> MRKYLEEKYNKFSLRKLTVGVCSMTIGSFFLVSTVQPEDYVVKAADNAIVHYKYVGEDNLTDKEKELIKKEVPSVVSSKEETYYLVFKPTKTTQLNKLPNTGLNYGVGSMLLGGMLGLVVVVVAKGKNKSRKILSILLVTSLGATTLELPARAMEDLQLSVYNMDYNLKVGDKLPEISSIPGYSFVGFIKNEAETKKENEEVKEQITSQQHNKKQPELKENTDENVIENKQENKTTLKISDKKEDKKVIENINKKDEKKVQGVNTVNPQDEVLAGKLTKPELLYSDKIIETPLKYNQIIESNDQLPEGTTRIKQQGKEGKKTEVIRMFTVEGKEVSRELISTKTEEPVSEIIEKGTKKAVSNVITKGQKLVKPAVEVKPEYTGVQAGAIVEPVKAEVPKEYTGVQAGAIVEPAKVETPKEYTGVQAGAIVEPAKAEVSKEYTGVQAGTIVEPAKAEVPKEYTGVQAGAIVEPEKVEPQYGGVTSGALVKPEKIEAPKEYTGVQAGAVVEPAKAEAPKEYRGVQAGAIVEPEKIESPKEYTGVQAGAVVEPAKAEVPKEYRGVQAGAIVEPEKIESPKEYTGEQSGAIVEPEKVETTKEYTGIQAGALVEPEKVEAPKEYTGVQAGAIVEPEKVEPPKEYTGVQAGAIVEPEKVEAPKEYTGKIEPLKTENPKPTVENNNTAEINNVPKNASALLRMNFVKGNQVLSGTGSATFIAPNVLLTVAHNFINNSADNSTGEFIGDKSKNTYEWQTPDGQKGSFTSEDIHFYNKKDYPKGFIYDLAVITLPQSTRRQHANLVENYSKVNVNDKLNVYGYPRGEYAHLKDTTVEIEQKYANNTYGVQYQGGKAGMSGGGIFNSKGEVIGLHQNGAENRSGGLILSPTQLDWIRSIIKGKEITPNYDALERHKDEKKDDIKEEKQVDKKLELRNISNVELYTLENNKYRHVSSLSSVPTNPEAYFMKVKSENFKDVMLPVKSIESARKDNQDVYKIVGQANDLIQHENNITLENYTYYLPKTVNSENGVYTSFKNLVDAMNINPYGTFRLGATMDAREVELSDGQESYINKEFSGKLIGENKGKYYAIYNLKKPLFKALSHATIQDLSIKEANVSSKEDAATIAKEAKNDTTIANVHSSGVIAGERSIGGLISQVTDSTISNSSFTGRITNTYDTTATYQIGGLVGKLSGVGALIEKSISSIDMATNANTGDQVVGGVAGVVDKKATIRNSYVEGNLNNVKPFGKVGGVVGNLWDRETSEVSNSGNLTNVLSDVNVTNGNAIAGYDFNGIKATNTYSNKNNKVVKVVQVDDEVLSKDSEEQRGTVLENNIVLEKKIELVPKKNTKIEDFNFSSRYETDYKNLKDADVSRLRVYKNIEKLLPFYNRETIVKYGNLVDANNTLYTKDLVSVVPMKDKEVISDINKNKTSINKLLLHYSDNTSQTLDIKYLQDFSKVAEYEIANTKLIYTPNTLLHSYNNIVKAVLNDLKSVQYDSDAVRKVLDISSNIKLTELYLDEQFTKTKANIEDSLSKLLSADAVIAENSNSIIDNYVIEKIKNNKEALLLGLTYLERWYNFKYDNTSAKDLVLYHLDFFGKSNSSALDNVIELGKSGFNNLLAKNNVITYNVLLSKNYGTEGLFKALEGYRKVFLPNVSNNDWFKTQSKAYIVEEKSTIPEVSSKQSKQGTEHSIGVYDRLTSPSWKYQSMVLPLLTLPEEKMIFMIANISTIGFGAYDRYRSSEYPKGDKLNRFVEENAQAAAKRFRDHYDYWYKILDKENKEKLFRSVLVYDAFRFGNDTNKETQEANFETNNPVIKNFFGPAGNNVVHNKHGAYATGDAFYYMAYRMLDKSGAVTYTHEMTHNSDREIYLGGYGRRSGLGPEFYAKGLLQAPDHSYD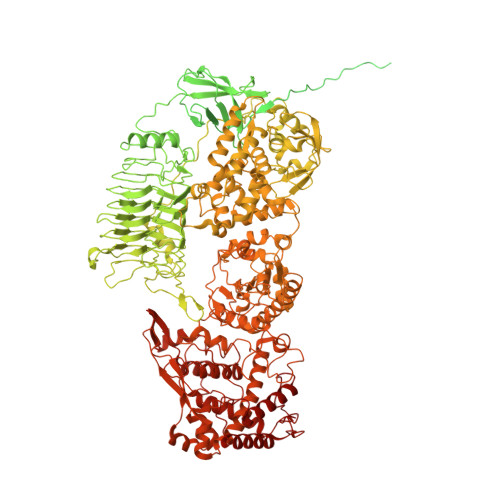PTITINSVLKYDDSENSTRLQIADPTQRFTNVEDLHNYMHNMFDLIYTLEILEGRAVAKLDYNEKNDLLRKIENIYKKDPDGNSVYATNAVRRLTSDEIKNLTSFDKLIENDVITRRGYIDQGEYERNGYHTINLFSPIYSALSSKIGTPGDLMGRRMAFELLAAKGYKEGMVPYISNQYEKEAKDRGSKIRSYGKEIGLVTDDLVLEKVFNKKYGSWVEFKKDMYKERVEQFSKLNRVSFFDPNGPWGRQKNVTVNNISVLEKMIETAVREDAEDFTAQVYPDTNSRVLKLKKAIFKAYLDQTKDFRTSIFGGK2-amino-2-deoxy-alpha-D-mannopyranose | C6 H13 N O5 | 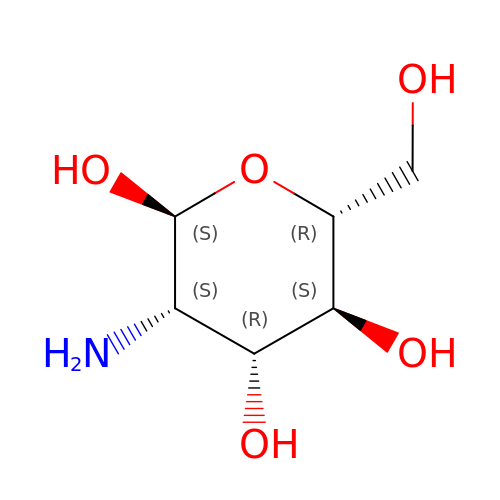MSWZFWKMSRAUBD-RXRWUWDJSA-N>MSESERLGIVRDFVAREILGREGILDSLADAPLALYERFAETGLMNWWVPKEHGGLGLGLEESVRIVSELAYGDAGVAFTLFLPVLTTSMIGWYGSEELKERFLGPLVARRGFCATLGSEHEAGSELARISTTVRRDGDTLVLDGTKAFSTSTDFARFLVVIARSADDPARYTAVTVPRDAPGLRVDKRWDVIGMRASATYQVSFSDCRVPGDNALNGN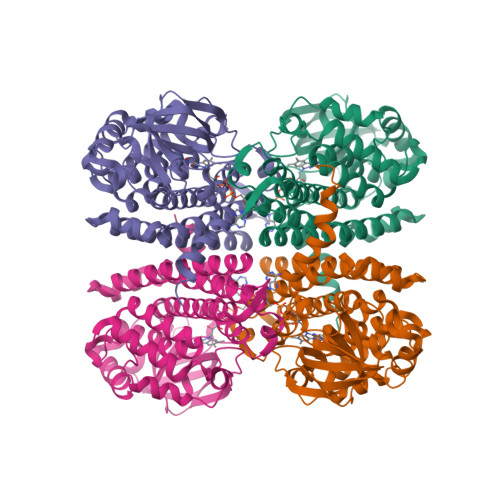GLRLLEIGLNASRILIAASALGVARRIRDVCMEYGKTKSLKGAPLVKDGVFAGRLGQFEMQIDVMANQCLAAARAYDATAARPDAARVLLRQGAQKSALTAKMFCGQTAWQIASTASEMFGGIGYTHDMVIGKLLRDVRHASIIEGGDDVLRDLVYQRFVVPTAKRTLEH[4x]>[2x]MLESKLKAPVFTATTQGDHYGEFVLEPLERGFGVTLGNPLRRILLSSIPGTAVTSVYIEDVLHEFSTIPGVKEDVVEIILNLKELVVRFLDPKMASTTLILRAEGPKEVRAGDFTPSADVEIMNPDLHIATLEEGGKLYMEVRVDRGVGYVPAERHGIKDRINAIPVDAIFSPVRRVAFQVEDTRLGQRTDLDKLTLRIWTDGSVTPLEALNQAVAILKEHLNYFANPEASLLPTPEVSKGEKRESAEEDLDLPLEELGLSTRVLHSLKEEGIESVRALLALNLKDLRNIPGIGERSLEEIRQALAKKGFTLKE;> MEIKRFGRIREVIPLPPLTEIQVESYKKALQADVPPEKRENVGIQAAFKETFPIEEGDKGKGGLVLDFLEYRIGDPPFSQDECREKDLTYQAPLYARLQLIHKDTGLIKEDEVFLGHLPLMTEDGSFIINGADRVIVSQIHRSPGVYFTPDPARPGRYIASIIPLPKRGPWIDLEVEASGVVTMKVNKRKFPLVLLLRVLGYDQETLVRELSAYGDLVQGLLDEAVLAMRPEEAMVRLFTLLRPGDPPKKDKALAYLFGLLADPKRYDLGEAGRYKAEEKLGVGLSGRTLVRFEDGEFKDEVFLPTLRYLFALTAGVPGHEVDDIDHLGNRRIRTVGELMADQFRVGLARLARGVRERMVMGSPDTLTPAKLVNSRPLEAALREFFSRSQLSQFKDETNPLSSLRHKRRISALGPGGLTRERAGFDVRDVHRTHYGRICPVETPEGANIGLITSLAAYARVDALGFIRTPYRRVKNGVVTEEVVYMTASEEDRYTIAQANTPLEGDRIATDRVVARRRGEPVIVAPEEVEFMDVSPKQVFSLNTNLIPFLEHDDANRALMGSNMQTQAVPLIRAQAPVVMTGLEERVVRDSLAALYAEEDGEVVKVDGTRIAVRYEDGRLVHPLRRYARSNQGTAFDQRPRVRVGQRVKKGDLLADGPASEEGFLALGQNVLVAIMPFDGYNFEDAIVISEELLKRDFYTSIHIERYEIEARDTKLGPERITRDIPHLSEAALRDLDEEGIVRIGAEVKPGDILVGRTSFKGEQEPSPEERLLRSIFGEKARDVKDTSLRVPPGEGGIVVGRLRLRRGDPGVELKPGVREVVRVFVAQKRKLQVGDKLANRHGNKGVVAKILPVEDMPHLPDGTPVDVILNPLGVPSRMNLGQILETHLGLAGYFLGQRYISPVFDGATEPEIKELLAEAFNLYFGKRQGEGFGVDKREKEVLARAEKLGLVSPGKSPEEQLKELFDLGKVVLYDGRTGEPFEGPIVVGQMFIMKLYHMVEDKMHARSTGPYSLITQQPLGGKAQFGGQRFGEMEVWALEAYGAAHTLQEMLTIKSD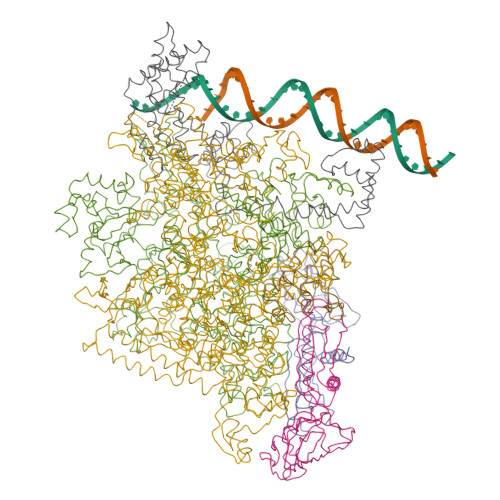DIEGRNAAYQAIIKGEDVPEPSVPESFRVLVKELQALALDVQTLDEKDNPVDIFEGLASKR;> MKKEVRKVRIALASPEKIRSWSYGEVEKPETINYRTLKPERDGLFDERIFGPIKDYECACGKYKRQRFEGKVCERCGVEVTRSIVRRYRMGHIELATPAAHIWFVKDVPSKIGTLLDLSATELEQVLYFNKYIVLDPKGAVLDGVPVEKRQLLTDEEYRELRYGKQETYPLPAGVDALVKDGEEVVKGQELAPGVVSRMDGVALYRFPRRVRVDYLRKERAALRIPLSAWVEKEAYRPGEVLAELSEPYLFRAEESGVVELKDLAEGHLIYLRQEEEVVARYFLPAGMTPLVVEGEIVEVGQPLAEGKGLLRLPRHMTAKEVEAEEEGDSVHLTLFLEWTEPKDYKVAPHMNVIVPEGAKVQAGEKIVAAIDPEEEVIAEAEGVVHLHEPASILVVKARVYPFEDDVEVTTGDRVAPGDVLADGGKVKSEIYGRVEVDLVRNVVRVVESYDIDARMGAEAIQELLKELDLEKLERELLEEMKHPSRARRAKARKRLEVVRAFLDSGNRPEWMILEAVPVLPPDLRPMVQVDGGRFATSDLNDLYRRLINRNNRLKKLLAQGAPEIIIRNEKRMLQEAVDAVIDNGRRGSPVTNPGSERPLRSLTDILSGKQGRFRQNLLGKRVDYSGRSVIVVGPQLKLHQCGLPKRMALELFKPFLLKKMEEKAFAPNVKAARRMLERQRDIKDEVWDALEEVIHGKVVLLNRAPTLHRLGIQAFQPVLVEGQSIQLHPLVCEAFNADFDGDQMAVHVPLSSFAQAEARIQMLSAHNLLSPASGEPLAKPSRDIILGLYYITQVRKEKKGAGMAFATPEEALAAYERGEVALNAPIVVAGRETSVGRLKFVFANPDEALLAVAHGLLDLQDVVTVRYLGRRLETSPGRILFARIVGEAVGDEKVAQELIQMDVPQEKNSLKDLVYQAFLRLGMEKTARLLDALKYYGFTLSTTSGITIGIDDAVIPEEKQRYLEEADRKLRQIEQAYEMGFLTDRERYDQVIQLWTETTEKVTQAVFKNFEENYPFNPLYVMAQSGARGNPQQIRQLCGMRGLMQKPSGETFEVPVRSSFREGLTVLEYFISSHGARKGGADTALRTADSGYLTRKLVDVAHEIVVREADCGTTNYISVPLFQMDEVTRTLRLRKRSDIESGLYGRVLAREVEALGRRLEEGRYLSLEDVHFLIKAAEAGEVREVPVRSPLTCQTRYGVCQKCYGYDLSMARPVSIGEAVGVVAAESIGEPGTQLTMRTFHTGGVAVGTDITQGLPRVIELFEARRPKAKAVISEIDGVVRIEEGEDRLSVFVESEGFSKEYKLPKDARLLVKDGDYVEAGQPLTRGAIDPHQLLEAKGPEAVERYLVDEIQKVYRAQGVKLHDKHIEIVVRQMLKYVEVTDPGDSRLLEGQVLEKWDVEALNERLIAEGKVPVAWKPLLMGVTKSALSTKSWLSAASFQNTTHVLTEAAIAGKKDELIGLKENVILGRLIPAGTGSDFVRFTQVVDQRTLKAIEEARKEAVEAKEKEAPRRPVRREQPGKGL;> MAEPGIDKLFGMVDSKYRLTVVVAKRAQQLLRHRFKNTVLEPEERPKMRTLEGLYDDPNAVTWAMKELLTGRLFFGENLVPEDRLQKEMERLYPTEEEA;> MKKSKSKKKAAKAQEVEVKEPVKEPEPLPELEAAEDLQDLPEPDPELLASEPELEDLADPLDLEGPLEADLLPEEGLLEEEEEELSLPKVSTSDPVRQYLHEIGQVPLLTLEEEIDLARKVEEGMEAIKKLSEATGLDQELIREVVRAKILGTARIQKIPGLKEKPDPKTVEEVDGKLKSLPKELKRYLHIAREGEAARQHLIEANLRLVVSIAKKYTGRGLSFLDLIQEGNQGLIRAVEKFEYKRRFKFSTYATWWIRQAINRAIADQARTIRIPVHMVETINKLSRTARQLQQELGREPSYEEIAEAMGPGWDAKRVEETLKIAQEPVSLETPIGDEKDSFYGDFIPDENLPSPVEAAAQSLLSEELEKALSKLSEREAMVLKLRKGLIDGREHTLEEVGAYFGVTRERIRQIENKALRKLKYHESRTRKLRDFLE>MAKVKIVGILNVTPNSFHDGGRFVETDKAVVRARELLSQGADIIEIGGESTGPGSNTITADEELARIVPVIRAIRSSLPDANIAVDTYKAEVARKALELGATMINDVSAGRADPKLFGVVARSNAQIVLMYSKDTDPHTSFDERQYVDVVRTVYDFLAERKKAAMSAGIPADRIILDTGLGGFVSSDPQYSFQLLAHLSDFQDLGCKLFLSPSRKSFLAGN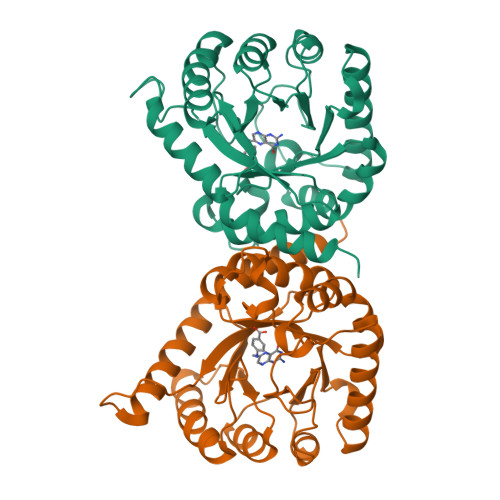ELLKTADRLPGTIAASAIAVLHGADYIRTHDVLEVRRGCEIATAINQPPER[2x]>[8x]MLAMSPPKPAVELDRHIDLDQAHAVASGGARIVLAPPARDRCRASEARLGAVIREARHVYGLTTGFGPLANRLISGENVRTLQANLVHFLASGVGPVLDWTTARAMVLARLVSIAQGASGASEGTIARLIDLLNSELAPAVPSRGTVGASGDLTPLAHMVLCLQGRGDFLDRDGTRLDGAEGLRRGRLQPLDLSHRDALALVNGTSAMTGIALVNAHACRHLGNWAVALTALLAECLRGRTEAWAAALSDLRPHPGQKDAAARLRARVDGSARVVRHVIAERRLDAGDIGTEPEAGQDAYSLRCAPQVLGAGFDTLAWHDRVLTIELNAVTDNP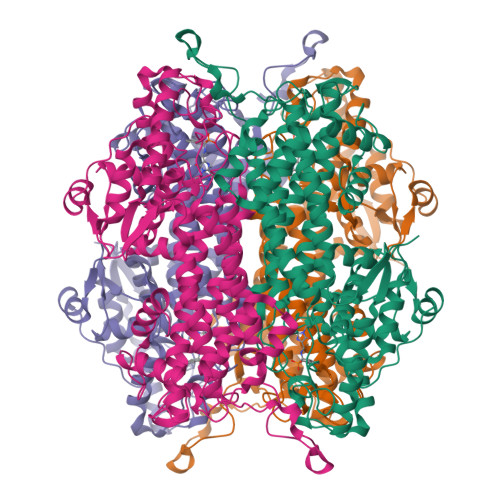VFPPDGSVPALHGGNFMGQHVALTSDALATAVTVLAGLAERQIARLTDERLNRGLPPFLHRGPAGLNSGFMGAQVTATALLAEMRATGPASIHSISTNAANQDVVSLGTIAARLCREKIDRWAEILAILALCLAQAAELRCGSGLDGVSPAGKKLVQALREQFPPLETDRPLGQEIAALATHLLQQSPV> TGGQQMGRGSEFDNITSDDHVVDTPGDTDNDHDGGEEPNPAYPLSDQSNEGDWVLNTEMSDEFELPL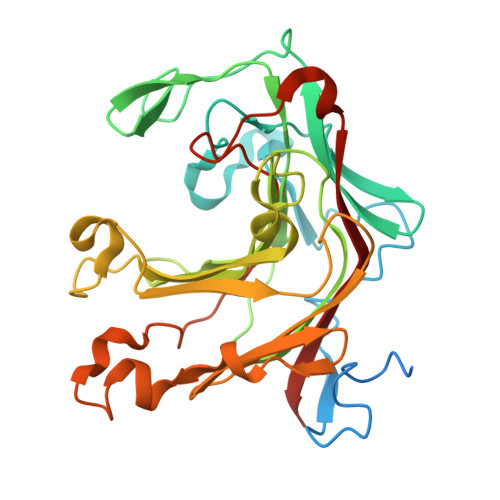DEDKWLIQGRNNEYQSRFIGRAPSQFSVNNAYTESGKLKIVTKWEPDYDFRLKFNGDDHDVVNGEKIYFENITTAAVISKKQFRYGYMEIKCKSANAPITSSFWTTGKNTSEMDMFEMFGGHKTNDSWRKRLKFNIISWDPNNPNYFNKINGPVFTQNIQVGNNTAGDFHVYGFDWTADYIKVYYDGVLLPEYTILKSELTNNNTNPDKWVTDSDYWIWFDSETFPWLGIPKEEDLPAEYQIEYLRVWQKNKIQ> SMIDDDGYRPNVGIVICNRQGQVMWARRFGQHSWQFPQGGINPGESAEQAMYRELFEEVGLSRKDVRILAS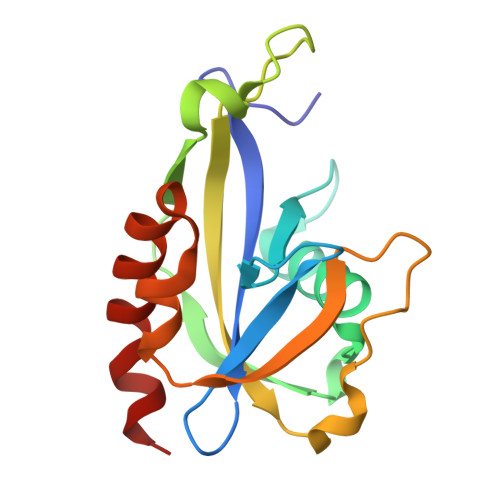TRNWLRYKLPKRLVRWDTKPVCIGQKQKWFLLQLVSGDAEINMQTSSTPEFDGWRWVSYWYPVRQVVSFKRDVYRRVMKEFASVVMSLA>MERAESSSTEPAKAIKPIDRKSVHQICSGQVVLSLSTAVKELVEN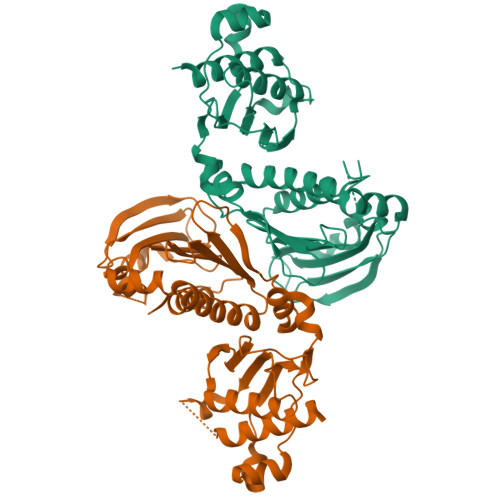SLDAGATNIDLKLKDYGVDLIEVSDNGCGVEEENFEGLTLKHHTSKIQEFADLTQVETFGFRGEALSSLCALSDVTISTCHASAKVGTRLMFDHNGKIIQKTPYPRPRGTTVSVQQLFSTLPVRHKEFQRNIKKEYAKMVQVLHAYCIISAGIRVSCTNQLGQGKRQPVVCTGGSPSIKENIGSVFGQKQLQSLIPFVQLPPSDSVCEEYGLSCSDALHNLFYISGFISQCTHGVGRSSTDRQFFFINRRPCDPAKVCRLVNEVYHMYNRHQYPFVVLNISVDSECVDISVTPDKRQILLQEEKLLLAVLKTSLIGMFDS[2x]>MAHAGRTGYDNREIVMKYIHYKLSQRGYEWDAGDDVEENRTEAPEGTESEVVHLTLRQAGDDFSRRYRRDFAEMSSQLHLTPFTARGRFATVVEELFRDGVNWGRIVAFFEFGGVMCVESVNREMSPLVD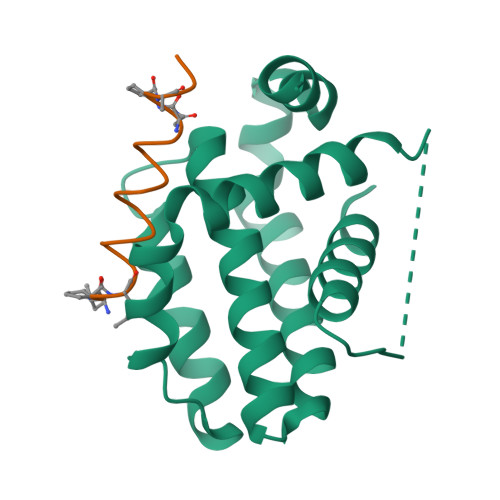NIALWMTEYLNRHLHTWIQDNGGWDAFVELYGPSMR[2x]>[2x]SNASERTGTQPLGVQGLTEEQRMMIRELMDAQMKTFDTTFSHFKNFRLPGVLSSGCELPESLQAPSREEAAKWSQVRKDLCSLKVSLQLRGEDGSVWNYKPPADSGGKEIFSLLPHMADMSTYMFKGIISFAKVISYFRDLPIEDQISLLKGAAFELCQLRFNTVFNAETGTWECGRLSYCLEDTAGGFQQLLLEPMLKFHYMLKKLQLHEEEYVLMQAISLFSPDRPGVLQHRVVDQLQEQFAITLKSYIECNRPQPAHRFLFLKIMAMLTELRSINAQHTQRLLRIQDIHPFATPLMQELFGITGSGGSGGSSHSSLTERHKILHRLLQEGSPS;>[2x]NEDMPVERILEAELAVEPKTETYVEANMGLNPSSPNDPVTNICQAADKQLFTLVEWAKRI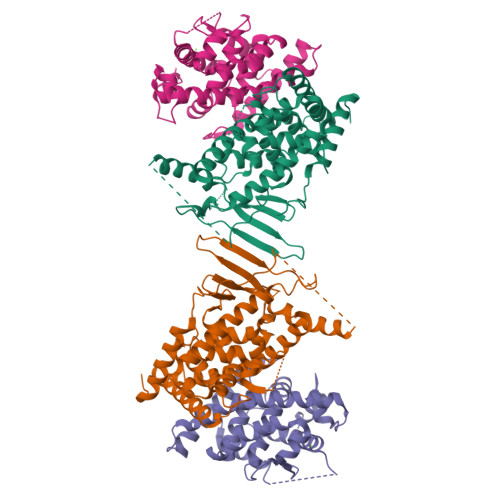PHFSELPLDDQVILLRAGWNELLIASFSHRSIAVKDGILLATGLHVHRNSAHSAGVGAIFDRVLTELVSKMRDMQMDKTELGCLRAIVLFNPDSKGLSNPAEVEALREKVYASLEAYCKHKYPEQPGRFAKLLLRLPALRSIGLKCLEHLFFFKLIGDTPIDTFLMEMLEAPHQMTGGSGGSSHSSLTERHKILHRLLQEGSPS>[2x]MKHHHHHHHMVSTLKPLKIGKHTIKFPIFQGGMGVGISWDELAGNVAKEGALGVISAVGTGYYKNMRFVERIVAKKPFEALNFYSKKALNEIFANARKICGNNPLGANILYAINDYGRVLRDSCEAGANIIITGAGLPTNMPEFAKDFSDVA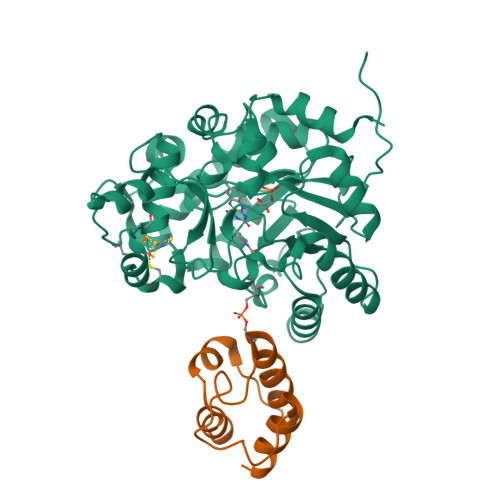LIPIISSAKALKILCKRWSDRYKRIPDAFIVEGPLSGGHQGFKYEDCFKEEFRLENLVPKVVEASKEWGNIPIIAAGGIWDRKDIDTMLSLGASGVQMATRFLGTKECDAKVYADLLPTLKKEDILLIKSPVGYPARAINTGVIKRIEEGNAPKIACVSNCVAPCNRGEEAKKVGYCIADGLGRSYLGNREEGLYFTGANGYRVDKIISVHELIKELTEG;>[2x]GTSSMGYLMALFEDIQAVIAEQLNVDAAQVTPEAEFVKDLGADSLDVVELIMALEEKFGIEIPDEQAEKIVNVGDVVKYIEDNKLA> CACACCG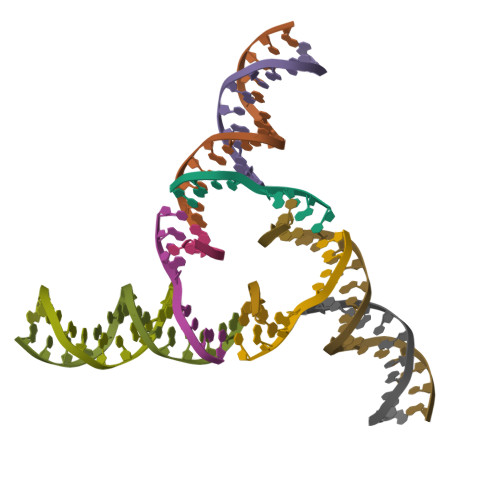T;> CTGTG;> ACGGACAGCACGTGCA;> GTGCACGTGCTGT> MSAG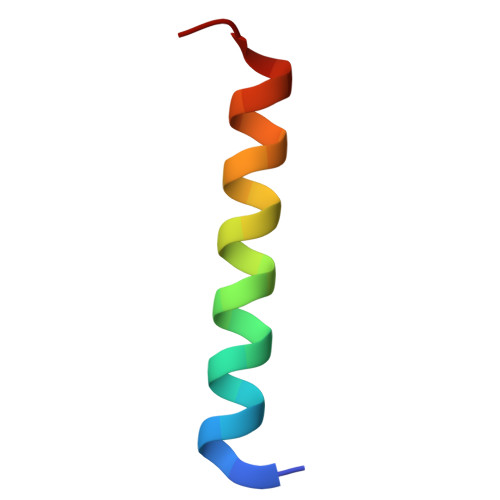VITGVLLVFLLLGYLVYALINAE> MASEVVSFSFTKFNPNPKDIILQGDALVTSKGKLQLTKVKDGKPVDHSLGRALYAAPIHIWDDSTDRVASFATSFSFVVEAP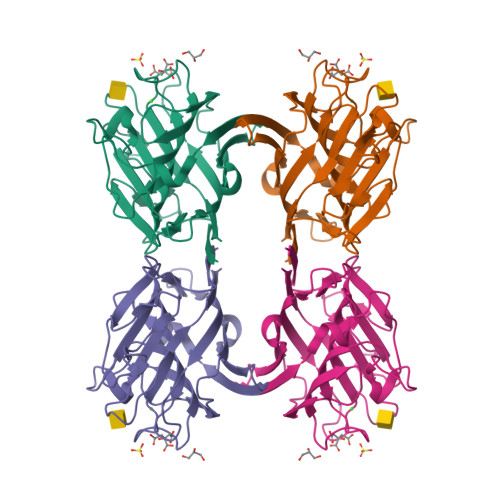DESKTADGIAFFLAPPDTQPQKDGGFLGLFNDSNKSIQTVAVEFDTFSNTWDPSARHIGINVNSIESMKYVKWGWENGKVANVYISYEASTKTLTASLTYPSNATSYIVSANVDLKSALPEWVRVGFSATSGLSRDHVETHDVLDWSFTSTLQAPSDDSNLEHHHHHH BIS-(N-ETHYLPYRIDINIUM-(3-METHOXYCARBAZOLE))HEXANE-1,6-DIAMINE | C42 H48 N6 O2 | 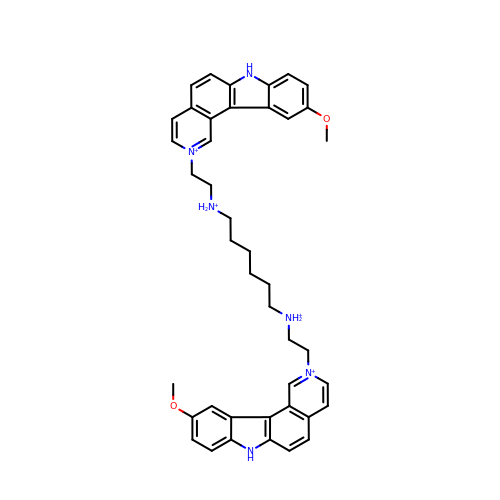VJZICIMRPZDSEJ-UHFFFAOYSA-R>[2x]MLPALIGISGH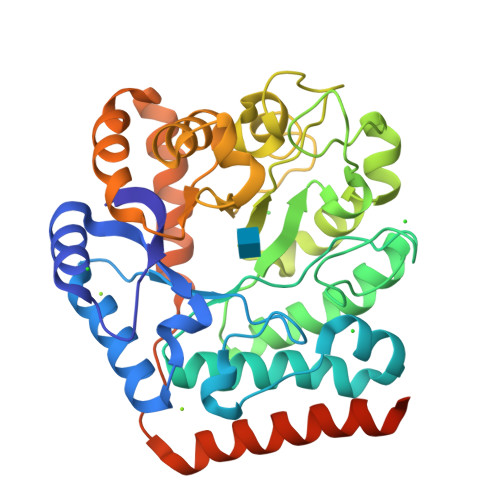EVGAEEEAAIRRLQPAGFILFSRNIDSVEQVRGLTESLRKLCLHHPVIAVDQEGGRVVRTASLGLNLPSPASLARLGSVGGIVELGAVTALALRYLGVNLNFAPVLDICHDPSAANALPGRCWGDNAQDVISRGGVYASNLRRGGVQSCGKHFPGMGRALADPHFSLPVIGLDERELFKTDLLPFLALCPALSSIMSAHIMLPQIDPDYPATLSERVIRGLLRDRLGFRGVVFTDDLCMGAITTQYSPDDAAFLSLKAGCDLPLICHDPLPWLDGLASRQESLNAYDRWDSFKRVEKLSDSLCFPFPEKASLWDSCLRRAEALCRLEEDGREKLPSSPVQKYLEHHHHHH>MDWHIAKHYDDILYYKAGGIAKIVINRPHKRNAFRPQTVFELYDAFCNAREDNRIGVVLLTGAGPHSDGKYAFCSGGDQSVRGEGGYIDDQGTPRLNVLDLQRLIRSMPKVVIALVAGYAIGGGHVLHLVCDLTIAADNAIFGQTGPKVGSFDGGFGSSYLARIVGQKKAREIWYLCRQYSAQEAERMGMVNTVVPVDRLEEEGIQWAKEILSKSPLAIRCLKAAFNADCDGQAGLQELAGNATLLYYMTEEG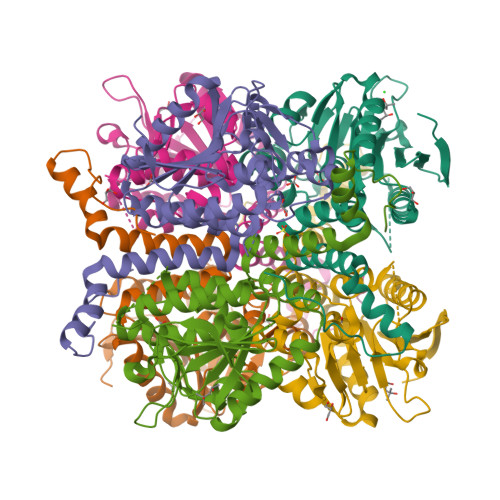SEGKQAFLEKRPPDFSQYPWLP[6x]> HHHHHHMIVLFVDFDYFYAQVEEVLNPSLKGKPVVVCVFSGRFEDSGAVATANYEARKFGVKAGIPIVEAKKILPNAVYLPMRKEVYQQVSSRIMNLLREYSEKIEIASIDEAYLDISDKVRDYREAYNLGLEIKNKILEKEKITVTVGISKNKVFAKIAADMAKPNGIKVIDDEEVKRLIRELDI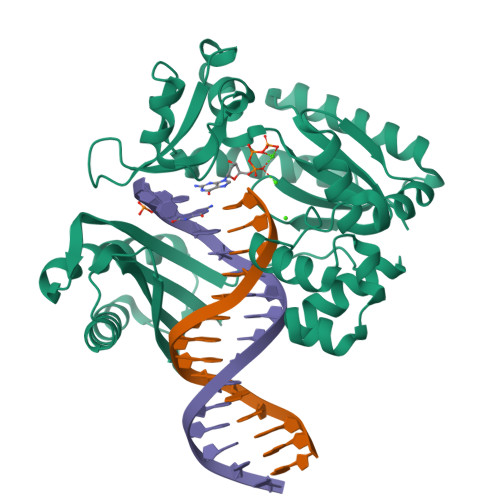ADVPGIGNITAEKLKKLGINKLVDTLSIEFDKLKGMIGEAKAKYLISLARDEYNEPIRTRVRKSIGRIVTMKRNSRNLEEIKPYLFRAIEESYYKLDKRIPKAIHVVAVTEDLDIVSRGRTFPHGISKETAYSESVKLLQKILEEDERKIRAIGVRFSKFIEAIGLDKFFDT1~{H}-indol-6-ylboronic acid | C8 H8 B N O2 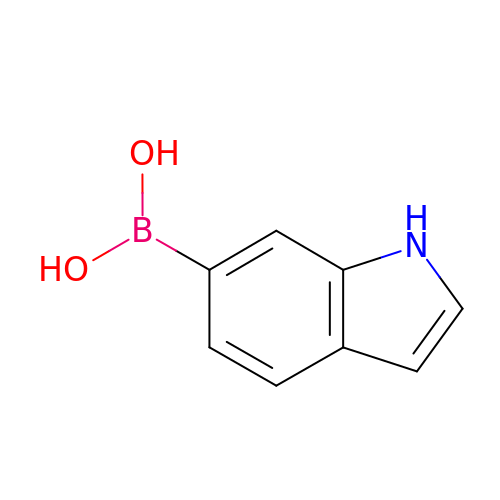| ZVMHOIWRCCZGPZ-UHFFFAOYSA-N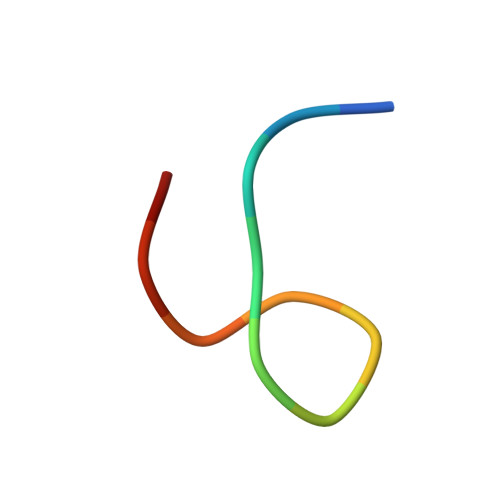> CWWKKKKKWWCA> GIEDLITEVAQGALTLSLPKQQDSLPDTKASGPAHSKEVPALTAVETGATNPLVPSDTVQTRHVIQRRSRSESTIESFFARGACVAIIEVDNEEPTTRAQKLFAMWRITYKDTVQLRRKLEFFTYSRFDMELTFVVTANFTNTNNGHALNQVYQIMYIPPGAPTPKSWDDYTWQTSSNPSIFYTYGAAPARISVPYVGLANAYSHFYDGFAKVPLKTDANDQIGDSLYSAMTVDDFGVLAIRVVNDHNPTKVTSKVRIYMKPKHVRVWCPRPPRAVPYYGPGVDYKDNLNPLSEKGLTTY;> MGAQVSSQKVGAHENSNRAYGGSTINYTTINYYKDSASNAASKQDYSQDPSKFTEPLKDVLIKTAPALNSPNVEACGYSDRVLQLTIGNSTITTQEAANSVVAYGRWPEFIRDDEANPVDQPTEPDVATCRFYTLDTVMWGKESKGWWWKLPDALRDMGLFGQNMYYHYLGRSGYTVHVQCNASKFHQGALGVFAIPEYCLAGDSDKQRYTSYANANPGEKGGKFYSQFNRDTAVTSPKREFCPVDYLLGCGVLLGNAFVYPHQIINLRTNNSATIVLPYVNAMAIDSMVKHNNWGIAILPLSPLDFAQESSVEIPITVTIAPMCSEFNGLRNVTAPKFQ;> GLPVLNTPGSNQYLTSDNYQSPCAIPEFDVTPPIDIPGEVKNMMELAEIDTMIPLNLENTKRNTMDMYRVTLSDSADLSQPILCFSLSPASDPRLSHTMLGEVLNYYTHWAGSLKFTFLFCGSMMATGKILVAYAPPGAQPPTSRKEAMLGTHVIWDLGLQSSCTMVVPWISNVTYRQTTQDSFTEGGYISMFYQTRIVVPLSTPKSMSMLGFVSACNDFSVRLLRDTTHISQSALPQ

The Enterovirus (EV) genus of the Picornaviridae family contains notable viral pathogens that cause various animal and human diseases and are regarded as potential zoonotic threats. These small non-enveloped RNA viruses contain 60 copies each of the viral proteins VP1-4 arranged to form an icosahedral protein capsid. VP1-3 each comprise a β-barrel with extended surface loops and C-termini that form the outer capsid surface. The N-termini of VP1-3, as well as the whole of VP4 (N-terminal to VP2 in the VP0 precursor), form a network on the inner surface. Glutathione (GSH), an important cellular reducing agent, is a crucial co-factor for the morphogenesis of enteroviruses, including PV.

Since PV3-SC8 has previously been shown to bind pocket factors such as GPP3 in the VP1 hydrophobic pocket, we investigated in situ if GSH binding interferes with this stabilisation mechanism by incubating a molar excess of GPP3 (VLP:compound molar ratio of 1:300) followed by GSH at 10 mM to form a ternary complex (PV3-SC8GPP3+GSH) with the PV3-SC8 VLP expressed in yeast. The cryo-EM electron potential map revealed the VP0, VP1 and VP3 capsid protein subunits of the PV3-SC8 VLP to be well ordered and there was an unambiguous feature for bound GSH in the interprotomer pocket formed between VP1 subunits from two adjacent protomers and VP3 from a single protomer; the same surface pocket shown to bind GSH in bovine enterovirus EVF330. The overall structure of the GSH-bound PV3-SC8 VLP is essentially identical to the unbound native antigenic form of PV3-SC8 VLP expressed previously in the plant, mammalian and yeast cells, with root-mean-square deviation (RMSD) in Cα atoms of 0.68, 1.39 and 0.77 Å, respectively. As expected GPP3 was observed bound within the hydrophobic pocket of VP1, in an essentially identical conformation to that previously observed for this compound bound to plant expressed PV3-SC818. This confirmed that the binding of GSH did not hinder the ability of the VP1 hydrophobic pocket to accommodate capsid-binding drugs such as GPP3, so effects at the two druggable sites, separated by some 22 Å in the capsid are likely to be additive. The GSH molecule observed bound in the VP1–VP3 surface pocket of the PV3-SC8 VLP is anchored in place by hydrogen bonds, salt-bridges and hydrophobic interactions. The carboxyl group of the GSH glycine moiety forms hydrogen bonds with two critical arginine residues; Arg257 and Arg242, contributed from neighbouring VP1 subunits of two capsid protomers. Additional hydrogen bonds are formed between Asp169 and Gln174 of VP1 with the amide and carbonyl oxygen groups of the cysteine moiety of GSH, respectively.> MAKWVYKFEEGNASMRNLLGGKGCNLAEMTILGMPIPQGFTVTTEACTEYYNSGKQITQEIQDQIFEAITWLEELNGKKFGDTEDPLLVSVRSAARASMPGMMDTILNLGLNDVAVEGFAKKTGNPRFAYDSYRRFIQMYSDVVMEVPKSHFEKIIDAMKEEKGVHFDTDLTADDLKELAEKFKAVYKEAMNGEEFPQEPKDQLMGAVKAVFRSWDNPRAIVYRRMNDIPGDWGTAVNVQTMVFGNKGETSGTGVAFTRNPSTGEKGIYGEYLINAQGEDVVAGVRTPQPITQLENDMPDCYKQFMDLAMKLEKHFRDMQDMEFTIEEGKLYFLQTRNGKRTAPAALQIACDLVDEGMITEEEAVVRIEAKSLDQLLHPTFNPAALKAGEVIGSALPASPGAAAGKVYFTADEAKAAHEKGERVI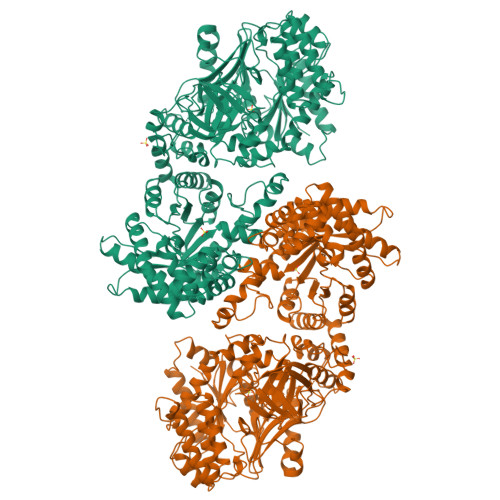LVRLETSPEDIEGMHAAEGILTVRGGMTSHAAVVARGMGTCCVSGCGEIKINEEAKTFELGGHTFAEGDYISLDGSTGKIYKGDIETQEASVSGSFERIMVWADKFRTLKVRTNADTPEDTLNAVKLGAEGIGLCRTEHMFFEADRIMKIRKMILSDSVEAREEALNELIPFQKGDFKAMYKALEGRPMTVRYLDPPLHEFVPHTEEEQAELAKNMGLTLAEVKAKVDELHEFNPMMGHRGCRLAVTYPEIAKMQTRAVMEAAIEVKEETGIDIVPEIMIPLVGEKKELKFVKDVVVEVAEQVKKEKGSDMQYHIGTMIEIPRAALTADAIAEEAEFFSFGTNDLTQMTFGFSRDDAGKFLDSYYKAKIYESDPFARLDQTGVGQLVEMAVKKGRQTRPGLKCGICGEHGGDPSSVEFCHKVGLNYVSCSPFRVPIARLAAAQAALNNK>HLTMPYVMPGDGEVVGVGEPVAIRFDENIADRGAAEKAIKITTNPPVEGAFYWLNNREVRWRPEHFWKPGTAVDVAVNT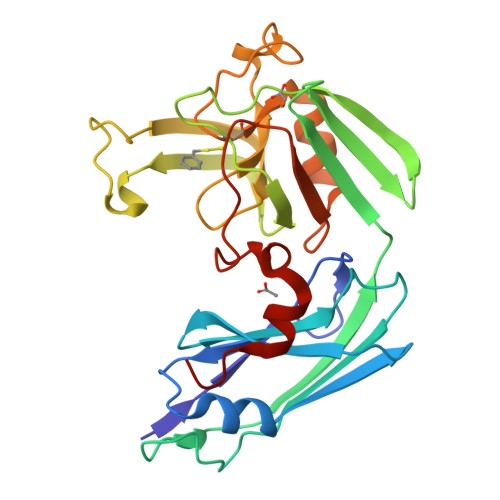YGVDLGEGMFGEDNVQTHFTIGDEVIATADDNTKILTVRVNGEVVKSMPTSMGKDSTPTANGIYIVGSRYKHIIMDSSTYGVPVNSPNGYRTDVDWATQISYSGVFVHSAPWSVGAQGHTNTSHGCLNVSPSNAQWFYDHVKRGDIVEVVNTVGGTLPGIDGLGDWNIPWDQWRAGNAKA[2x]ADENOSINE-2'-MONOPHOSPHATE 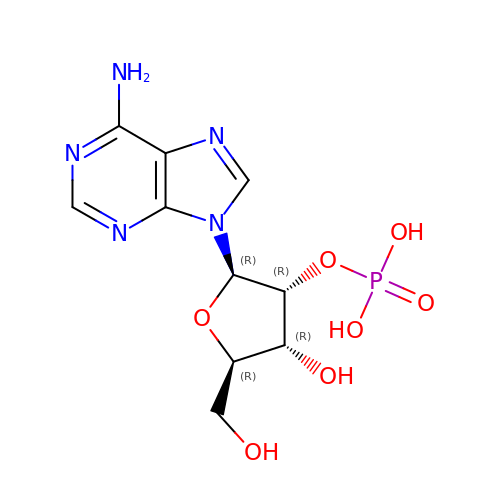| C10 H14 N5 O7 P | QDFHPFSBQFLLSW-KQYNXXCUSA-N> GSTGLIKHTEYMEFLKSVPTFQSLPEEILSKLADVL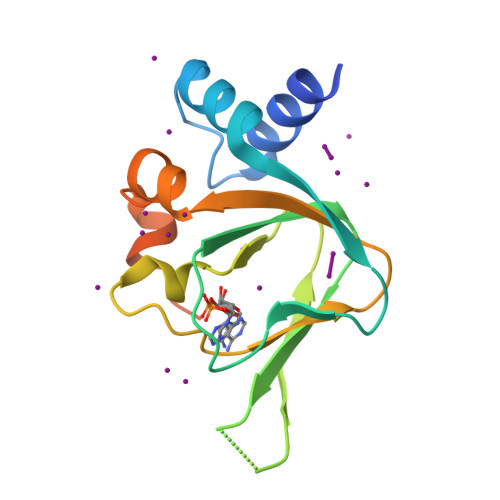EETHYENGEYIIRQGARGDTFFIISKGTVNVTREDSPSEDPVFLRTLGKGDWFGEKALQGEDVRTANVIAAEAVTCLVIDRDSFKHLIGGLDDVSNKAYEDAEAKAKYEAEAAFFAN> GLHCPSDWYYYDQHCYRIFNEEMNWEDAEWFCTKQAKGAHLVSIKSAKEADF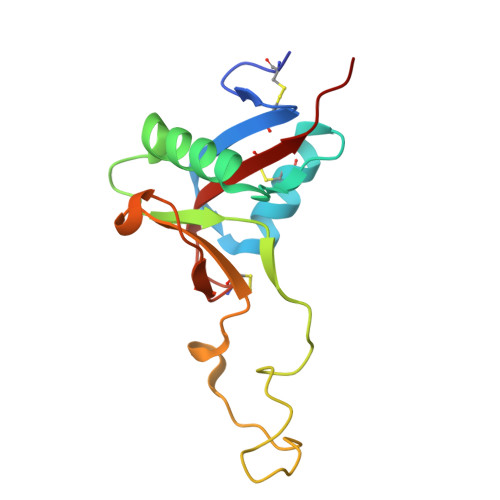VAWMVTQNIEESFSHVSIGLRVQNKEKQCSTKWSDGSSVSYDNLLDLYITKCSLLKKETGFRKWFVASCIGKIPFVCKFPPQC> GPLGSMSEEQVAQDTEEVFRSYVFYRHQQEQEAEGVAAPADPEMVTL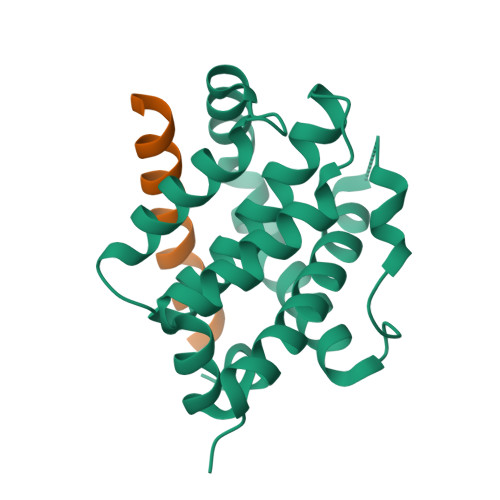PLQPSSTMGQVGRQLAIIGDDINRRYDSEFQTMLQHLQPTAENAYEYFTKIATSLFESGINWGRVVALLGFGYRLALHVYQHGLTGFLGQVTRFVVDFMLHHSIARWIAQRGGWVAALNLGNG;> XAPYLEQVARTLRKIGEEINEALRX> GDTKHEVRHENP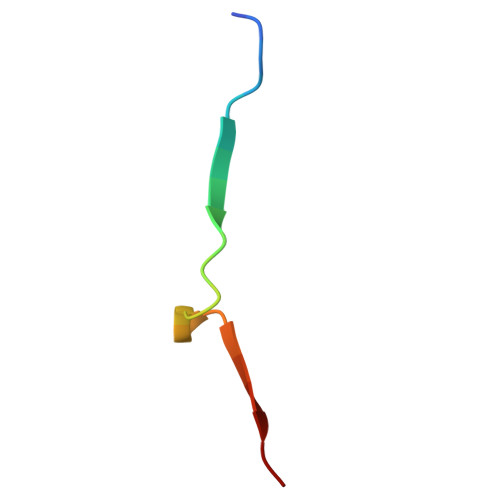QDEAQTIVVNK> EWEALEKKLAALESKCQALE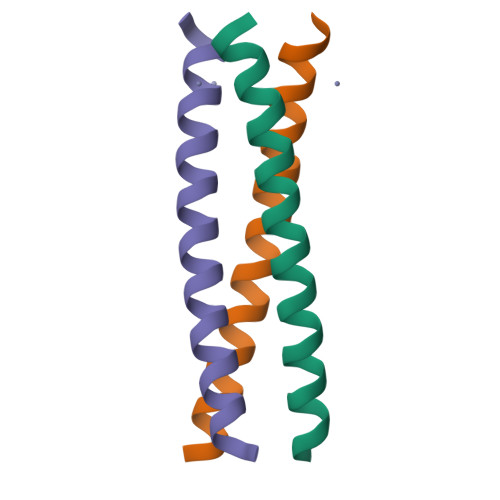KKCQALEKKLEALEHG> MAHHHHHHVDDDDKENLYFQMKGKVQKILIWKWGQPPSPTPVPRPPDADPNTPSPKPLEGRPERQF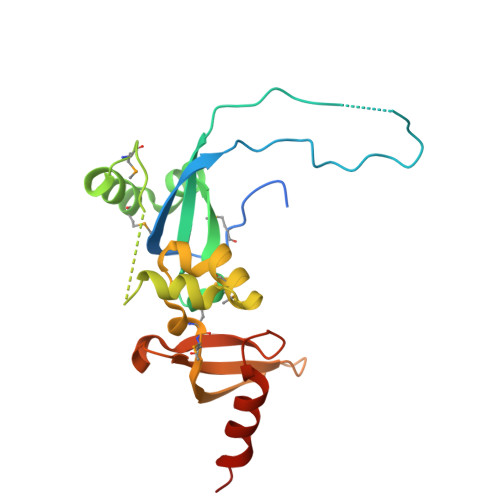FVKWQGMSYWHCSWVSELQLELHCQVMFRNYQRKNDMDEPPSGDFGGDEEKSRKRKNKDPKFAEMEERFYRYGIKPEWMMIHRILNHSVDKKGHVHYLIKWRDLPYDQASWESEDVEIQDYDLFKQSYWNHRELKK>MVSGVGGSGGGRGGGRGGEEEPSSSHTPNNRRGGEQAQSSGTKSLRPRSNTESMSKAIQQYTVDARLHAVFEQSGESGKSFDYSQSLKTTTYGSSVPEQQITAYLSRIQRGGYIQPFGCMIAVDESSFRIIGYSENAREMLGIMPQSVPTLEKPEILAMGTDVRSLFTSSSSILLERAFVAREITLLNPVWIHSKNTGKPFYAILHRIDVGVVIDLEPARTEDPALSIAGAVQSQKLAVRAISQLQALPGGDIKLLCDTVVESVRDLTGYDRVMVHKFHEDEHGEVVAESKRDDLEPYIGLHYPATDIPQASRFLFKQNRVRMIVDCNATPVLVVQDDRLTQSMCLVGSTLRAPHGCHSQYMANMGSIASLAMAVIINGNEDDGSNVASGRSSMRLWGLVVCHHTSSRCIPFPLRYACEFLMQAFGLQLNMELQLALQMSEKRVLRTQTLLCDMLLRDSPAGIVTQSPSIMDLVKCDGAAFLYHGKYYPLGVAPSEVQIKDVVEWLLANHADSTGLSTDSLGDAGYPGAAALGDAVCGMAVAYITKRDFLFWFRSHTAKEIKWGGAKHHPEDKDDGQRMHPRSSFQAFLEVVKSRSQPWETAEMDAIHSLQLILRDSFKESEAAMNSKVVDGVVQPCRDMAGEQGIDELGAVAREMVRLIETATVPIFAVDAGGCINGWNAKIAELTGLSVEEAMGKSLVSDLIYKENEATVNKLLSRALRGDEEKNVEVKLKTFSPELQGKAVFVVVNACSSKDYLNNIVGVCFVGQDVTSQKIVMDKFINIQGDYKAIVHSPNPLIPPIFAADENTCCLEWNMAMEKLTGWSRSEVIGKMIVGEVFGSCCMLKGPDALTKFMIVLHNAIGGQDTDKFPFPFFDRNGKFVQALLTANKRVSLEGKVIGAFCFLQIP[2x];> MMFLPTDYCCRLSDQEYMELVFENGQILAKGQRSNVSLHNQRTKSIMDLYEAEYNEDFMKSIIHGGGGAITNLGDTQVVPQSHVAAAHETNMLESNKHVDDSETLKASSSKRMMVDYHNRKKIKFIPPDEQSVVADRSFKLGFDTSSVGFTEDSEGSMYLSSSLDDESDDARPQVPARTRK

The red/far-red light receptor phytochrome B (phyB) plays essential roles in regulating various plant development processes. PhyB exists in two distinct photoreversible forms: the inactive Pr form and the active Pfr form. phyB-Pfr binds phytochrome-interacting factors (PIFs) to transduce red light signals. PhyB covalently binds the linear tetrapyrrole PΦB as a chromophore. In these structures, two parallel phyB-Pfr molecules interact with one PIF6 molecule.

In this study, we determined the cryo-EM structures of the photoactivated Arabidopsis phyB-Pfr‒PIF6 complex, the constitutively active mutant phyBY276H‒PIF6 complex, and the HKRD-truncated phyBNY276H‒PIF6 complex. We tested the interactions between PIF6β and phyBNY276H, red light-irradiated phyBN, or the HKRD region. Pull-down and SEC results revealed that phyBNY276H and red light-irradiated phyBN interact with PIF6β, but the HKRD region cannot interact with PIF6β, confirming that phyBN is sufficient for PIF6β binding. Only the PSMs of each phyBNY276H protomer and the N-terminal region of PIF6β (PIF6N) are clearly modeled, but the PAS1 and PAS2 domains could not be modeled due to the absence of density maps. Structural alignment revealed that the structures of the full-length phyBY276H‒PIF6β complex and the phyBNY276H‒PIF6β complex are nearly identical (r.m.s.d. of 0.657 Å over 966 Cα atoms). The PΦB molecules adopt a “Z” configuration in both structures.> GSHMKTCVPADINKEEEFVEEFNRLKTFANFPSGSPVSASTLARAGFLYTGEGDTVRCFSCHAAVDRWQYGDSAVGRHRKVSPNCRFINGFYLE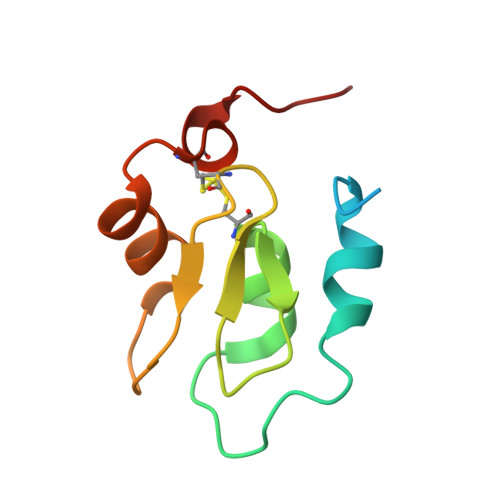N> SHTDIKVPNFSDYRRPPDDYSTKSSRESDPSRKGFSYLVTAVTTLGVAYAAKNVVTQFVSSMSASADVLAMSKIEIKLSDIPEGKNMAFKWRGKP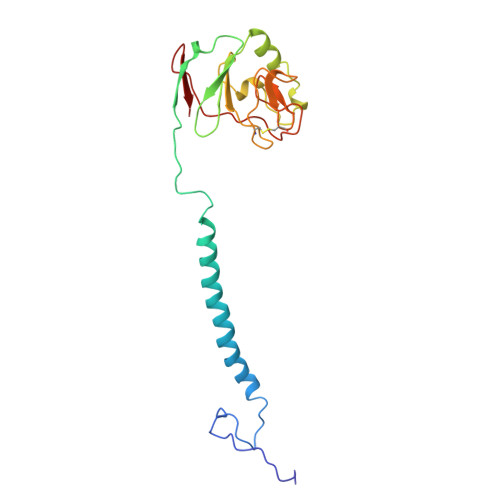LFVRHRTKKEIDQEAAVEVSQLRDPQHDLERVKKPEWVILIGVCTHLGCVPIANAGDFGGYYCPCHGSHYDASGRIRKGPAPLNLEVPSYEFTSDDMVIVG>[2x]GPQMLSANERLKNNFNILYNQIRQYPAYYFKVASNVPTYSDICQSFSVMYQGFQIVNHSGDVFIHACRENPQSKGDFVGDKFHISIAREQ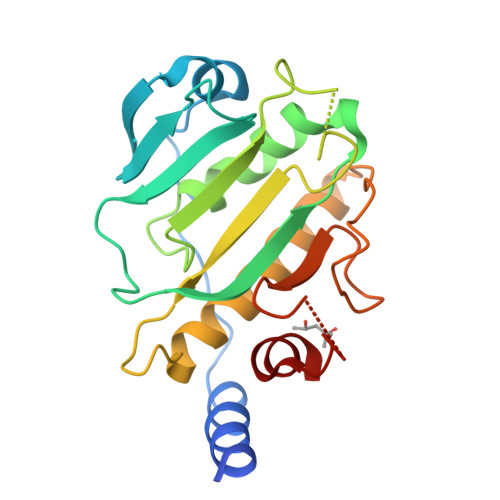VPLAFQILSGLLFSEDSPIDKWKITDMNRVSQQSRVGIGAQFTLYVKSDQECSQYSALLLHKIRQFIMCLESNLLRSKIAPGEYPASDVRPEDWKYVSYRNELRSDRDGSERQEQMLREEPFYRLMIE> MEIGVPKEIKNQEFRVGLSPSSVRTLVEAGHTVFIETQAGIGAGFADQDYVQAGAQVVPSAKDAWSREMVVKVKEPLPAEYDLMQKDQLLFTYLHLAAARELTEQLMRVGLTAIAYETVELPNRSLPLL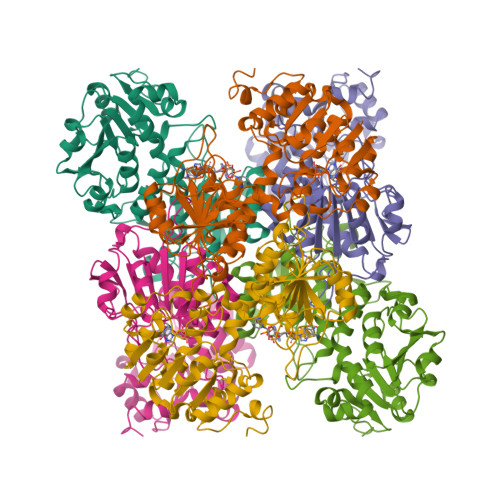TPMSIIAGRLSVQFGARFLERQQGGRGVLLGGVPGVKPGKVVILGGGVVGTEAAKMAVGLGAQVQIFDINVERLSYLETLFGSRVELLYSNSAEIETAVAEADLLIGAVLVPGRRAPILVPASLVEQMRTGSVIVDVAVDQGGCVETLHPTSHTQPTYEVFGVVHYGVPNMPGAVPWTATQALNNSTLPYVVKLANQGLKALETDDALAKGLNVQAHRLVHPAVQQVFPDLA>[2x]KISPIETVPVKLKPGMDGPKVKQWPLTEEKIKALVEICTEMEKEGKISKIGPENPYNTPVFAIKKKDSTKWRKLVDFRELNKRTQDFWEVQLGIPHPAGLKKKKSVTVLDVGDAYFSVPLDEDFRKYTAFTIPSINNETPGIRYQYNVLPQGWKGSPAIFQSSMTKILEPFRKQNPDIVIYQYMDDLYVGSDLEIGQHRTKIEELRQHLLRWGLTTPDKKHQKEPPFLWMGYELH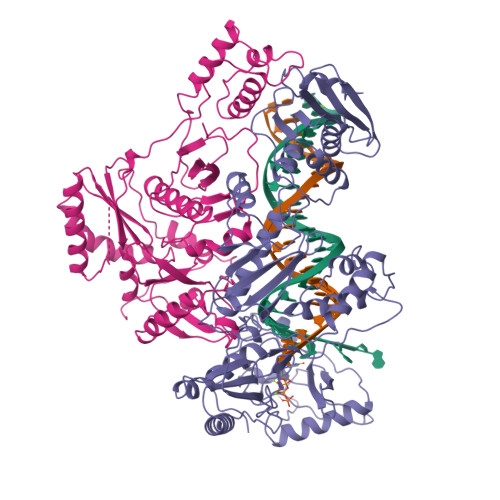PDKWTVQPIVLPEKDSWTVNDICKLVGKLNWASQIYPGIKVRQLCKLLRGTKALTEVIPLTEEAELELAENREILKEPVHGVYYDPSKDLIAEIQKQGQGQWTYQIYQEPFKNLKTGKYARMRGAHTNDVKQLTEAVQKITTESIVIWGKTPKFKLPIQKETWETWWTEYWQATWIPEWEFVNTPPLVKLWYQLEKEPIVGAETFYVDGAANRETKLGKAGYVTNKGRQKVVPLTDTTNQKTQLQAIYLALQDSGLEVNIVTDSQYALGIIQAQPDESESELVNQIIEQLIKKEKVYLAWVPAHKGIGGNEQVDKLVSA;>[2x]PISPIETVPVKLKPGMDGPKVKQWPLTEEKIKALVEICTEMEKEGKISKIGPENPYNTPVFAIKKKDSTKWRKLVDFRELNKRTQDFWEVQLGIPHPAGLKKKKSVTVLDVGDAYFSVPLDEDFRKYTAFTIPSINNETPGIRYQYNVLPQGWKGSPAIFQSSMTKILEPFRKQNPDIVIYQYMDDLYVGSDLEIGQHRTKIEELRQHLLRWGLTTPDKKHQKEPPFLWMGYELHPDKWTVQPIVLPEKDSWTVNDIQKLVGKLNWASQIYPGIKVRQLCKLLRGTKALTEVIPLTEEAELELAENREILKEPVHGVYYDPSKDLIAEIQKQGQGQWTYQIYQEPFKNLKTGKYARMRGAHTNDVKQLTEAVQKITTESIVIWGKTPKFKLPIQKETWETWWTEYWQATWIPEWEFVNTPPLVKLWYQLEKEPIVGAETF> MDGSGEQPRGGGPTSSEQIMKTGALLLQGFIQDRAGRMGGEAPELALDPVPQDASTKKLSESLKRIGDELDSNMELQRMIAAVDTDSPREVFFRVAADMFSDGNFNWGRVVALFYFASKLVLKALSTKVPELIRTIMGW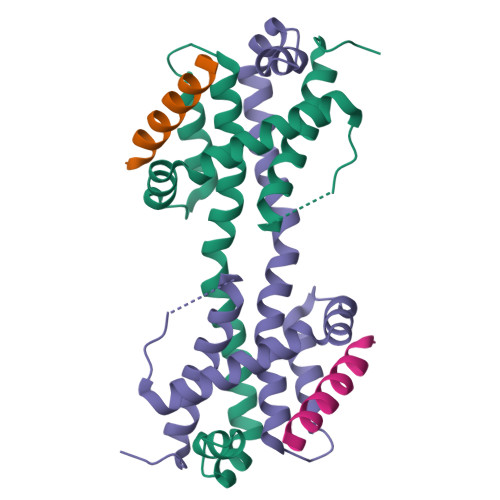TLDFLRERLLGWIQDQGGWDGLLSYFGTPTWQGSS;> DPVPQDASTKKLSECLKRIGDELDSNMELQRMIA N-[(1R)-1-borono-3-methylbutyl]-Nalpha-(pyrazine-2-carbonyl)-D-phenylalaninamide 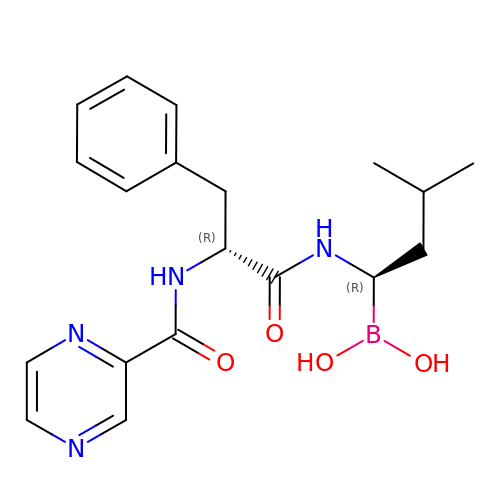| C19 H25 B N4 O4 | GXJABQQUPOEUTA-WBVHZDCISA-N> PSTGSKPSAPPQDISCTSPSSTSILVSWQPPPVEKQNGIITEYSI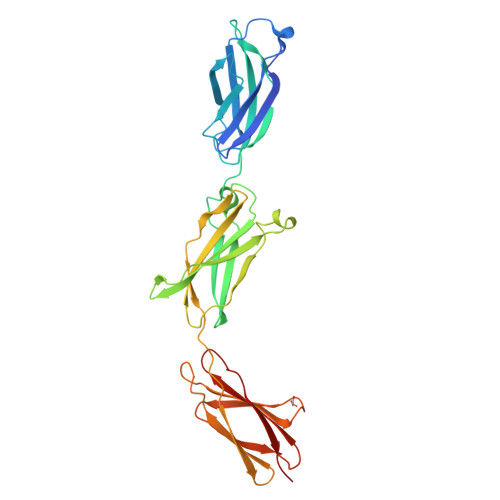KYTAVDGEDDKPHEILGIPSDTTKYLLEQLEKWTEYRITVTAHTDVGPGPESLSVLIRTNEDVPSGPPRKVEVEAVNSTSVKVSWRSPVPNKQHGQIRGYQVHYVRMENGEPKGQPMLKDVMLADAQWEFDDTTEHDMIISGLQPETSYSLTVTAYTTKGDGARSKPKLVSTTGAVPGKPRLVINHTQMNTALIQWHPPVDTFGPLQGYRLKFGRKDMEPLTTLEFSEKEDHFTATDIHKGASYVFRLSARNKVGFGEEMVKEISIPEE>MSGMRVYLGADHAGYELKQRIIEHLKQTGHEPIDCGALRYDADDDYPAFCIAAATRTVADPGSLGIVLGGSGNGEQIAANKVPGARCALAWSVQTAALAREHNNAQLIGIGGRMHTVAEALAI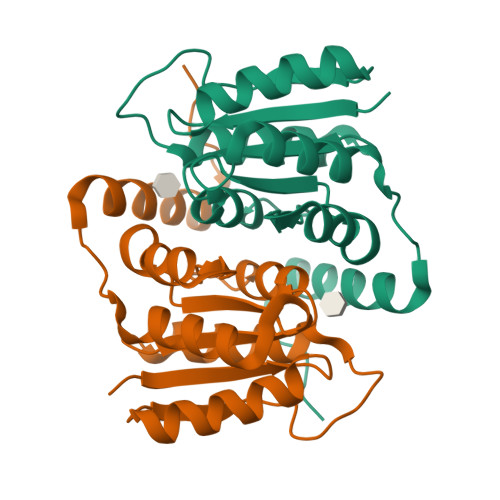VDAFVTTPWSKAQRHQRRIDILAEYERTHEAPPVPGAPA[5x]1-methyl-3-naphthalen-2-yl-1H-pyrazolo[3,4-d]pyrimidin-4-amine 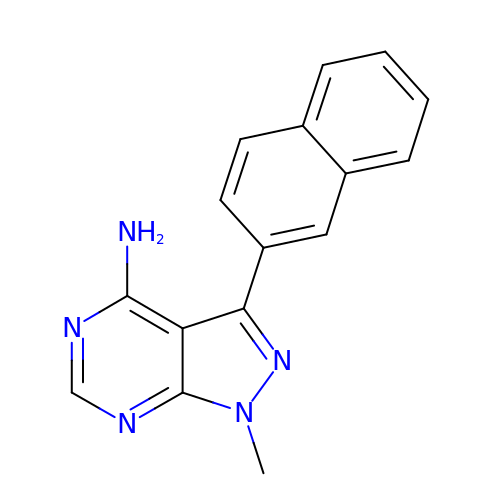| C16 H13 N5 | UOKGZPYGRJDACN-UHFFFAOYSA-N>[2x]STNDDPLTPLNRFDKYYLRMFKKVPRLQQNGSNIINGVNMKNTVIVLYFFAKWCQACTMQSTEMD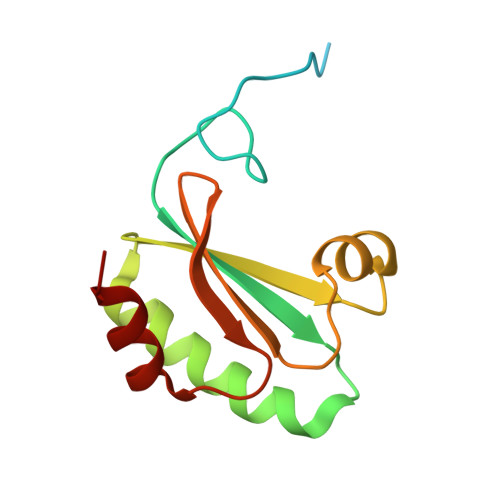KLQKYYGKRIYLLKVDLDKNESLARKFSVKSLPTIILLKNKTMLARKDHFVSSNDLIALIKKH> MDYMERPKLGLIVREPYASLIVDGRKVWEIRRRKTRHRGPLGIVSGGRLIGQADLVGVEGPFSVEELLAHQEKHLAEEAFLRAYAKDEPLYAWVLENAFRYEKPLHVPRRPGRVMFVDLSE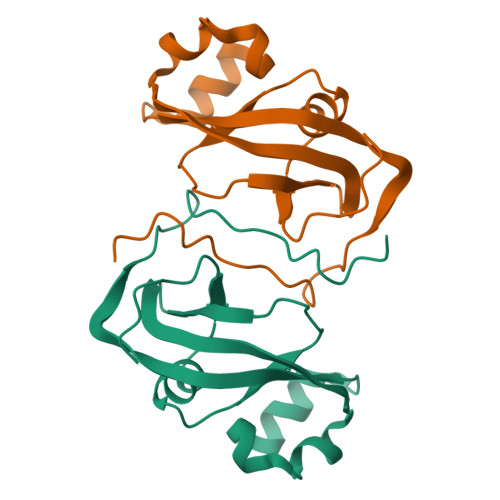VRW> GENLYFQGMRCIGMSNRDFVEGVSGGSWVDIVLEHGSCVTTMAKNKPTLDFELIKTEAKQPATLRKYCIEAKLTNTTTESRCPTQGEPSLNEEQDKRFVCKHSMVDRGWGNGCGLFGKGGIVTCAMFRCKKNMEGKVVQPENLEYTIVITPHSGEEHAVGNDTGKHGKEIKITPQSSITEAELTGYGTVTMECSPRTGLDFNEMVLLQMENKAWLVHRQWFLDLPLPWLPGADTQGSNWIQKETLVTFKNPHAKKQDVVV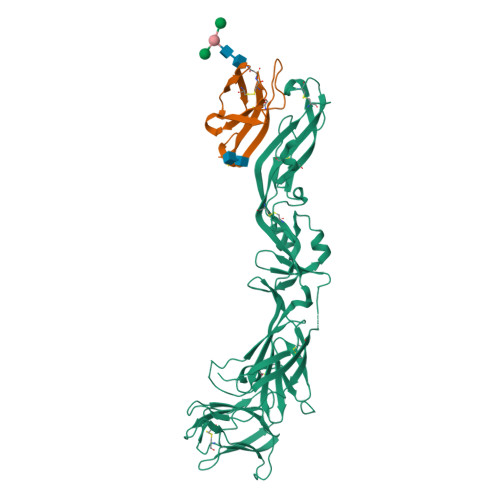LGSQEGAMHTALTGATEIQMSSGNLLFTGHLKCRLRMDKLQLKGMSYSMCTGKFKVVKEIAETQHGTIVIRVQYEGDGSPCKIPFEIMDLEKRHVLGRLITVNPIVTEKDSPVNIEAEPPFGDSYIIIGVEPGQLKLNWFKK;> FHLTTRNGEPHMIVSRQEKGKSLLFKTEDGVNMCTLMAMDLGELCEDTITYKCPLLRQNEPEDIDCWCNSTSTWVTYGTCTTMGEHSTEKSSVALVPHVGMGLETRTETWMSSEGAWKHVQRIETWILRH>GSGGSGGITEAQARAIVNSALKLYSQDKTGMVDFALESGGGSILSTRCSETYETKTALMSLFGIPLWYFSQSPRVVIQPDIYPGNCWAFKGSQGYLVVRLSMMIHPAAFTLEHIPKTLSPTGNISSAPKDFAVYGLENEYQEEGQLLGQFT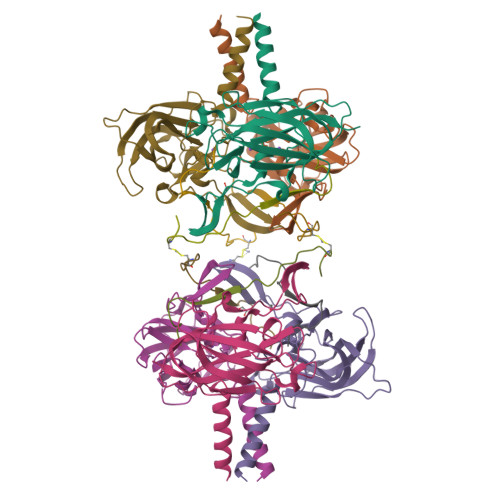YDQDGESLQMFQALKRPDDTAFQIVELRIFSNWGHPEYTCLYRFRVHGEPVK[6x];>[6x]GSMASGGPCCSHARIPRTPYLVLSYVNGLPPV>[2x]EAEAKTFTRCSLAREMYKLGVPKNQLARW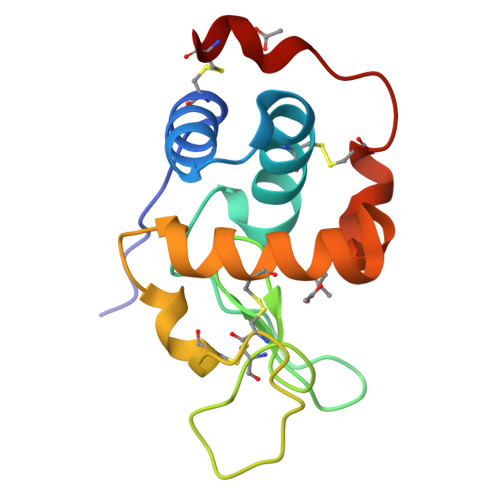TCIAEHESSYNTKAVGSLNSNGSRDYGIFQINNYYWCSPPSGAFSYDECKIKCEDFLVDSIEPAVKCAQLVLKQQGWTAWSTWKYCDGTLPSIDDCF> KKPKNKDKDKKVPEPDNKKKKPKKEEEQKWKWWEEERYPEGIKWKFLEHKGPVFAPPYEPLPENVKFYYDGKVMKLSPKAEEVATFFAKMLDHEYTTKEIFRKNFFKDWRKEMTNEEKNIITNLSKCDFTQMSQYFKAQTEARKQMSKEEKLKIKEENEKLLKEYGFCI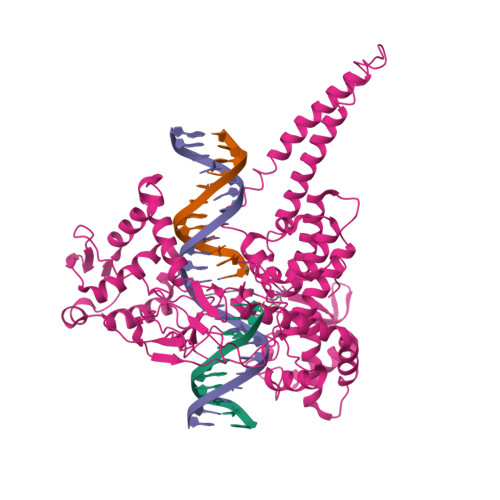MDNHKERIANFKIEPPGLFRGRGNHPKMGMLKRRIMPEDIIINCSKDAKVPSPPPGHKWKEVRHDNKVTWLVSWTENIQGSIKYIMLNPSSRIKGEKDWQKYETARRLKKCVDKIRNQYREDWKSKEMKVRQRAVALYFIDKLALRAGNEKEEGETADTVGCCSLRVEHINLHPELDGQEYVVEFDFLGKDSIRYYNKVPVEKRVFKNLQLFMENKQPEDDLFDRLNTGILNKHLQDLMEGLTAKVFRTYNASITLQQQLKELTAPDENIPAKILSYNRANRAVAILCNHQRAPPKTFEKSMMNLQTKIDAKKEQLADARRDLKSAKADAKVMKDAKTKKVVESKKKAVQRLEEQLMKLEVQATDREENKQIALGTSKLNYLDPRITVAWCKKWGVPIEKIYNKTQREKFAWAIDMADEDYEF> QYSPNTQQGRTSIVHLFEWRWVDIALECERYLAPKGFGGVQVSPPNENVAIYNPFRPWWERYQPVSYKLCTRSGNEDEFRNMVTRCNNVGVRIYVDAVINHMCGNAVSAGTSSTCGSYFNPGSRDFPAVPYSGWDFNDGKCKTGSGDIENYNDATQVRDCRLTGLLDLALEKDYVRSKIAEYMNHLIDIGVAGFRLAASKHMW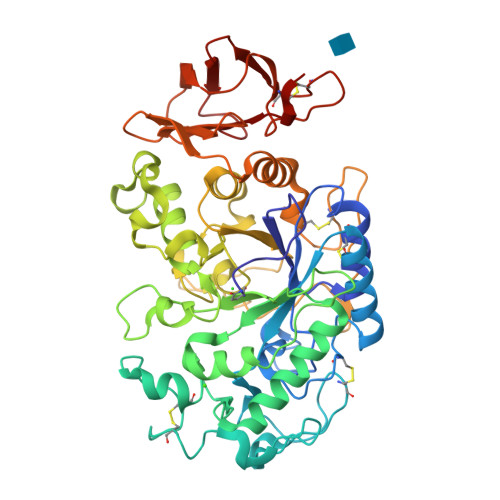PGDIKAILDKLHNLNSNWFPAGSKPFIYQEVIDLGGEPIKSSDYFGNGRVTEFKYGAKLGTVIRKWNGEKMSYLKNWGEGWGFVPSDRALVFVDNHDNQRGHGAGGASILTFWDARLYKMAVGFMLAHPYGFTRVMSSYRWPRQFQNGNDVNDWVGPPNNNGVIKEVTINPDTTCGNDWVCEHRWRQIRNMVIFRNVVDGQPFTNWYDNGSNQVAFGRGNRGFIVFNNDDWSFSLTLQTGLPAGTYCDVISGDKINGNCTGIKIYVSDDGKAHFSISNSAEDPFIAIHAESKL> ADPQAGSLDLQIDEEQPAGTLIGDISAGLPAGTAAPLMYFISAQEGSGVGTDLAIDEHSGVVRTARVLDREQRDRYRFTAVTPDGATVEVTVRVADI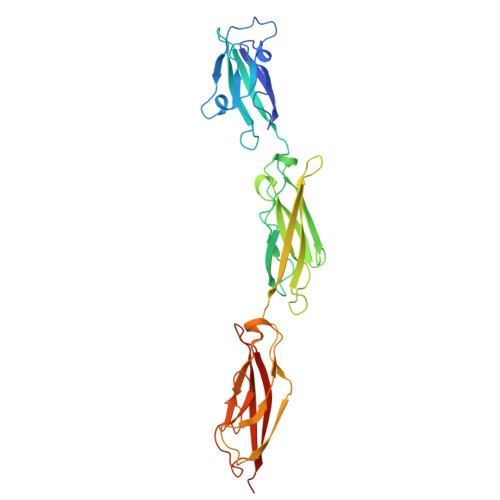NDHAPAFPQARAALQVPEHTAFGTRYPLEPARDADAGRLGTQGYALSGDGAGETFRLETRPGPDGTPVPELVVTGELDRENRSHYMLQLEAYDGGSPPRRAQALLDVTLLDINDHAPAFNQSRYHAVVSESLAPGSPVLQVFASDADAGVNGAVTYEINRRQSEGDGPFSIDAHTGLLQLERPLDFEQRRVHELVVQARDGGAHPELGSAFVTVHVRDAN>MGGSSGGGVSYRSGGESDVELEDYEVDDFRDGIVESRGNRFNPLTNFLGLDFAGGSGGKFTVINGIRDISRGSI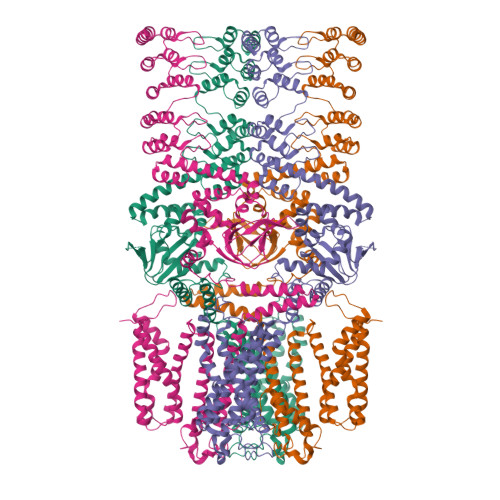VHPDNRWYKAWTMFILIWALYSSFFTPLEFGFFRGLPENLFILDIAGQIAFLVDIVLTFFVAYRDSRTYRMIYKRSSIALRYLKSTFIIDLLACMPWDIIYKAAGEKEEVRYLLLIRLYRVHRVILFFHKMEKDIRINYLFTRIVKLIFVELYCTHTAACIFYYLATTLPASQEGYTWIGSLKLGDYSYSKFREIDPWTRYTTSMYFAVVTMATVGYGDIHAVNMREMIFAMVYISFNMILGAYLIGNMTALIVKGSKTERFRDKMADIMRYMNRNKLGRNIRGQITGHLRLQYESSYTEAAVLQDIPVSIRAKIAQTLYLPYIEKVPLFRGCSSEFINQIVIRLHEEFFLPGEVIMEQGSVVDQLYFVCHGVLEEIGITKDGSEEIVAVLQPDHSFGEISILCNIPQPYTVRVAELCRILRLDKQSFMNILEIFFHDGRRILNNLLEGKESNVRIKQLESDITFHISKQEAELALKLNSAAFYGDLYQLKSLIRAGGDPNKTDYDGRSPLHLAASRGYEDITLYLIQESVDVNIKDKLGSTPLLEAIKNGNDRVAALLVKEGATLNIENAGTFLCTVVAKGDSDFLKRLLSNGIDPNSKDYDHRTPLHVAASEGFYVLAIQLVEASANVLAKDRWGNTPLDEALGCGNKMLIKLLEDAKNSQISSFPSGSKEPKDKVYKKKCTVYFSHPGDSKEKRRRGIVLWVPRSIEELIRTAKEQLNVPEASCVLSEDEAKIIDVDLISDGQKLYLAVET[4x]>AIDEIKSRGYLLVGLSADFPPFEFVDENGNIVGFDVDLAKEIARRLGVELKIVDMTFDGLIPSLLTKKIDVIISGMTITEERKKVVAFSDPYFDAGQVIVVRKDSDFRPKTYEDLVGKTVAVQIGTTGDIEVSKYDGIKVVRFDKFTDAFLELKRGRADAVVLDSATARAFVAKNPDLVISSGVLSSEQYGIAVRKEDTDLLEFINSVLRELKKSPYDVLIEKWFSE[2x]

We identified the arginine binding protein form Thermatoga maritima (TmArgBP) as an ideal system for arginine detection. Additionally, in contrast to the vast majority of SBP that operate as monomers, TmArgBP forms multimeric assemblies at room temperature. The secondary structural elements and protein organization in distinct subdomains (lobes) connected by two joining fragments confirm that TmArgBP is a type II SBP. One novel element emerged from the present study is that the protein forms a dimer through the swapping of the C-terminal helix.

The structure of the apo form was solved by performing multi-wavelength anomalous diffraction experiments, collecting data at three distinct wavelengths. The structure solution unveils the presence of two independent polypeptide chains in the asymmetric unit of the ApoTmArgBP crystals. An analysis of the intermolecular contacts established by ApoTmArgBP molecules within the crystals, carried out by using the server PISA, clearly indicates that the these two independent molecules constitute a stable dimer. Indeed, the total buried area in the complex is 1387 Å2. Similar to other arginine-binding proteins, ApoTmArgBP is folded into two distinct lobes, each consisting of a β-sheet core formed by five strands, surrounded by helices. β-sheets of lobes I (residues 23–110 and residues 210–231) and II (residues 116–203) present topologies β2β1β3β5β4 and β8β7β9β6β10, respectively. In line with unliganded SBPs, the two lobes of the proteins are far away from each other and do not establish significant non-covalent interactions. Indeed, the two subunits in the dimer mutually exchange their C-terminal helix (residues 237–246). An important role in the swapping process is played by the hinge region 232-KKSPY-236 whose extended conformation hampers the association of the terminal helix with its own subunit and favors its anchoring the main body of the other polypeptide chain. Using the program DynDom, we computed a difference in the closure angle between lobe I and lobe II of 20° for the apo form, whereas no difference was detected for the holo form. Indeed, the C-terminal helix of Apo-TmArgBP forms interactions with residues at the closed interface between the two lobes of the adjacent monomer, an interface which is not accessible in the Holo form, since locked by the arginine ligand.3-[[8-(1-methylindol-6-yl)quinoxalin-6-yl]amino]-~{N}-[(3~{S})-1-methylpiperidin-3-yl]pyridine-4-carboxamide 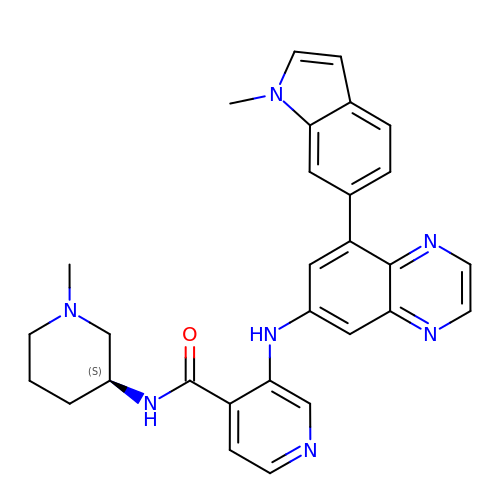| C29 H29 N7 O | CZIVVJNETCQZQP-NRFANRHFSA-N Methyl N-[4-[5-chloro-2-[[3-[5-chloro-2-(tetrazol-1-yl)phenyl]propanoylamino]methyl]-1H-imidazol-4-yl]phenyl]carbamate | C22 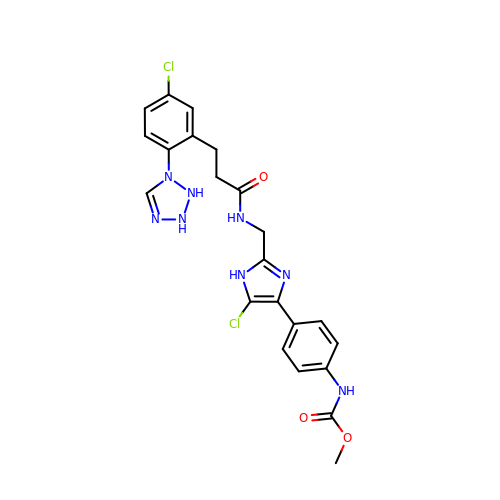H22 Cl2 N8 O3 | JTVUNKGTKMZKDP-UHFFFAOYSA-N>[2x]HHHHHHIEGRGAYVLDDSDGLGREFDGIGAVSGGGATSRLLVNYPEPYRSEILDYLFKPNFGASLHILKVEIGGDGQTTDGTEPSHMHYELDENYFRGYEWWLMKEAKKRNPDIILMGLPWSFPGWLGKGFSWPYVNLQLTAYYVVRWILGAKHYHDLDIDYIGIWNERPFDANYIKELRKMLDYQGLQRVRIIASDNLWEPISSSLLLDQELWKVVDVIGAHYPGTYTVWNAKMSGKKLWSSEDFSTINSNVGAGCWSRILNQNYINGNMTSTIAWNLVASYYEELPYGRSGLMTAQEPWSGHYVVASPIWVSAHTTQFTQPGWYYLKTVGHLEKGGSYVALTDGLGNLTIIIETMSHQHSMCIRPYLPYYNVSHQLAT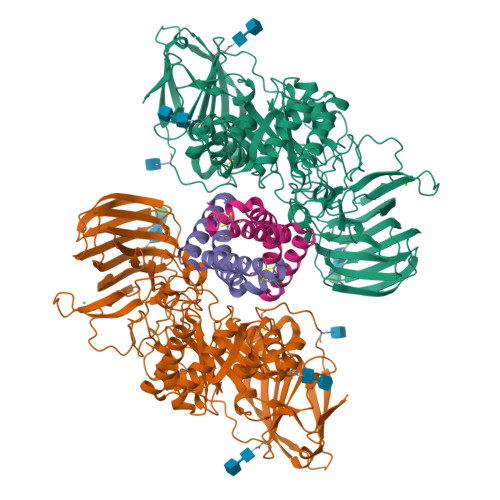FTLKGSLREIQELQVWYTKLGTPQQRLHFKQLDTLWLLDGSGSFTLELEEDEIFTLTTLTTGRKGSYPPPPSSKPFPTNYKDDFNVEYPLFSEAPNFADQTGVFEYYMNNEDREHRFTLRQVLNQRPITWAADASSTISVIGDHHWTNMTVQCDVYIETPRSGGVFIAGRVNKGGILIRSATGVFFWIFANGSYRVTADLGGWITYASGHADVTAKRWYTLTLGIKGYFAFGMLNGTILWKNVRVKYPGHGWAAIGTHTFEFAQFDNFRVEAAR;>MGKSLPCDICKTVVTEAGNLLKDNATQEEILHYLEKTCEWIHDSSLSASCKEVVDSYLPVILDMIKGEMSNPGEVCSALNLCQSLQE[2x]RV is a non-enveloped double-stranded RNA (dsRNA) virus with three concentric capsid layers encapsidating eleven dsRNA segments. The outermost layer contains the glycoprotein VP7 and the protease-sensitive spike protein VP4, which define the classification of RVs into G and P genotypes, respectively. RVs use the VP8* domain of the spike protein VP4 to recognize specific host glycans in a genotype-dependent manner. Our studies show that VP8* of these genotypes engages the type I precursor glycan (Galβ1,3-GlcNAc) at a unique and conserved binding site that is present in all P, P and P HRVs, and the subtle sequence and structural changes lead to an altered glycan configuration at the reducing end in the neonate-specific P RV, that may play a key role in the age-restricted tropism of some P strains.

The P VP8* in our X-ray crystallography and NMR studies is from the neonate-specific HRV vaccine strain RV3. To understand how the VP8* of neonate-specific P HRV recognizes type I glycans, we determined the structure of P VP8* with H-type I pentasaccharide (also known as Lacto-N-fucopentaose I or LNFP1) at the resolution of 1.8 Å. Distinct from the HBGA binding sites in P and P HRVs or the Sia-binding site in ARVs, the H-type I glycan binding site consists of one of the β-sheets and the C-terminal α-helix of P VP8*. The residues L167, W174, T184, T185, R209, and E212 are involved either in hydrophobic interactions or in a network of direct or water-mediated hydrogen bond interactions with type I precursor Galβ1,3-GlcNAc at the non-reducing end. The Gal4 moiety interacts with R209 and H169 via hydrophobic and hydrogen bonding interactions, and also in hydrophobic interactions with Y170 and W174. The reducing end of the H-type I glycan is further stabilized through a set of interactions between the Glc5 moiety with the residues H169, N171, S172, W174, and Y187. In the complex structures, the sidechains of Y170 and N171 change orientation to engage in a hydrophobic interaction with Gal4 and a hydrogen bond interaction with Glc5 of the glycan, respectively. In addition, the side chain of R209, that forms a hydrogen bond with E212 in the apo structure, binds to GlcNAc via hydrogen bond and hydrophobic interactions in the structure of P VP8*/H-type I complex. As a result of the rotational changes in the glycosidic bond in the neonate-specific P VP8*, the reducing end of the glycan is brought closer to VP8* establishing a number of hydrophobic interactions involving Y170, N171, and Y187 and hydrogen bond interactions involving N171 and S172. Remarkably in the neonatal P VP8*, a single residue H169, which is well conserved in most neonate-specific [P6] genotypes, alters the conformation of the glycan to sterically restrict branching at the reducing end.

> GSLDGPYQSTSFKPPSDYWILLNPTNQQVVLEGTNKTDIWVALLLVEPNVTNQSRQYTLFGETKQITVENNTNKWKFFEMFRSSVSAEFQHKRTLTSDTKLAGFLKHYNSVWTFHGETPHATTDYSSTSNLSEVETTIHVEFYIIPRSQESKCVEYINTGL>[2x]SNAMFLINGHAQDQLAVSDRATQFGDGSFTTARIVDGNICHLEAHLQRLQVACEKLRIAFSHWSTLR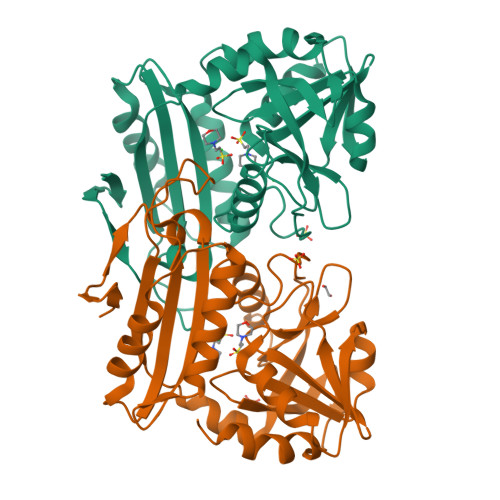QEMTMLATGHDSGVLKVIISRGSGGRGYSAMNCQAATRILSVSAYPAYYSQWRKQGITLTLSPIPLGRNPYLAGLKHLNRLEQVLIRSHLEQTDADEALVLDSEGWVTECCAANLFWRTGDIVFTPRLDQAGVNGIMRQFCLRQLAQSPFQVLEVQAREEAVRQADEIIICNALMPIIPIRAYHGTSYSSRTLFQFLAPFCEHPN>VDAGLDQIENREVLRPLLEALPERERTVLVLRFFDSMTQTQIAERVGISQMHVSRLLAKSLARLRDQLE[3x];>[3x]MADLNWMQRGVRAVELNVAARLENLALLRTLVGAIGTFEDLDFDAVADLRLAVDEVCTRLIRSALPDATLRLVVDPRKDEVVVEASAACDT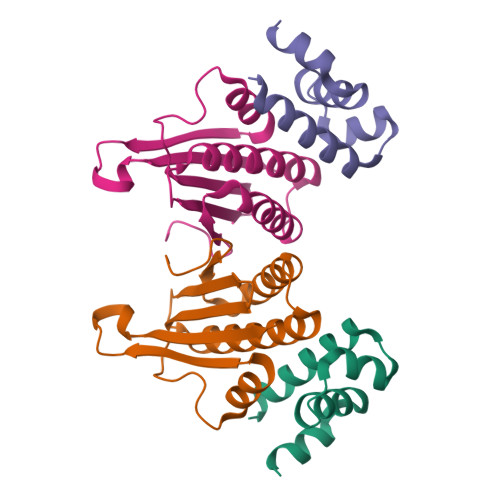HDVVAPGSFSWHVLTALADDVQTFHDGRQPDVAGSVFGITLTARRAASSR>[2x]VIHYSSGKDLCPVKGWAPLSKDNGIRIGSRGEVFVIREPFISCSINECRTFFLTQGALLNDKHSNGTVKDRSPFRTLMSCPIGVAPSPSNSRFESVAWSATACSDGPGWLTIGITGPDATAVAVLKYNGIITDTLKSWKGNIMRTQESECVCQDEFCYTLITDGPSDAQAFYKILKIKKGKIVSVKDVDAPGFHFEECSCYPSGENVECVCR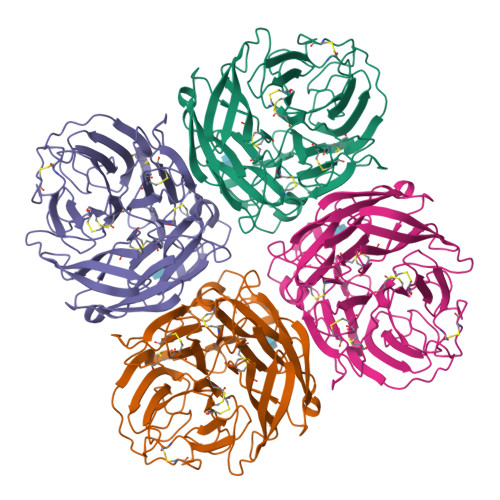DNWRGSNRPWIRFNSDLDYQIGYVCSGVFGDNPRPMDSTGSCNSPINNGKGRYGVKGFSFRYGDGVWIGRTKSLESRSGFEMVWDANGWVSTDKDSNGVQDIIDNDNWSGYSGSFSIRGETTGRNCTVPCFWVEMIRGQPKEKTIWTSGSSIAFCGVNSDTTGWSWPDGALLPFDIDK>PPGPPGPPGERGPPGGVGFPGPPGPPGPPG[6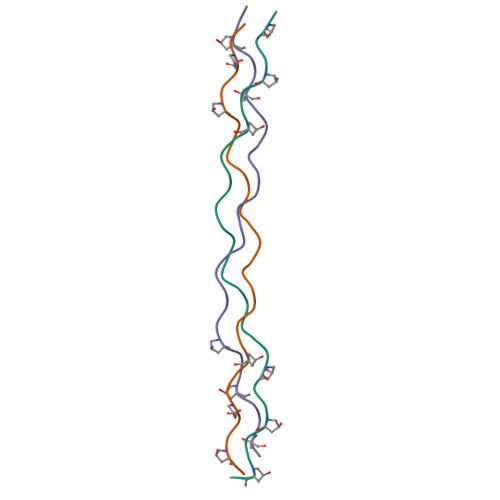x]>MRGSHHHHHHGMASMPLHHLTRFPRLEFIGAPTPLEYLPRLSDYLGREIYIKRDDVTPIAMGGNKLRKLEFLVADALREGADTLITAGAIQSNHVRQTAAVAAKLGLHCVALLENPIGTTAENYLTNGNRLLLDLFNTQIEMCDALTDPDAQLQTLATRIEAQGFRPYVIPVGGSSALGAMGYVESALEIAQQCEEVVGLSSVVVASGSAGTHAGLAVGLEHLMPDVELIGVTVSRSVAEQKPKVIALQQAIAGQLALTATADIHLWDDYFAPGYGVPNDAGMEAVKLLASLEGVLLDPVYTGKAMAGLIDGISQKRFNDDGPILFIHTGGAPALFAYHPHV[8x]

D-cysteine (D-Cys) moieties are found in firefly luciferin, semisynthetic cephalosporin MT141 and malformin A. D-cysteine desulfhydrase (DCyD) is suggested to take part in the catabolic degradation of D-Cys and D-Cys-containing toxic compounds. The polypeptide fold of StDCyD is similar to those of other fold type II PLP-dependent enzymes and consists of a small domain (residues 48–161) and a large domain (residues 1–47 and 162–328). As in other PLP-dependent fold type II enzymes, the active site is situated in a large crevice between the two domains. StDCyD is specific for D-Cys and βCDA, and shows no activity with ACC, although it shares significant sequence identity with ACCDs.

Structures of two distinct crystal forms of recombinant StDCyD were determined by the molecular replacement method. In the form I structure, there are two dimers (AB and CD) and in form II structure, there are four dimers (AB, CD, EF and GH) in the asymmetric unit that are similar to the dimeric organization found in other fold type II PLP-dependent enzymes. Electron density map of unliganded StDCyD revealed a significant patch of density with tetrahedral geometry at the active site that could be interpreted as a sulphate (in form I crystal structure) or a phosphate (in form II crystal structure). Form I crystals were obtained in a condition which had sulphate while conditions for obtaining form II had phosphate ions. These ions could be refined to reasonable B factors that were close to those of the surrounding atoms. Therefore, Form II structure has been utilized only for qualitative analysis.> QQIEQPYR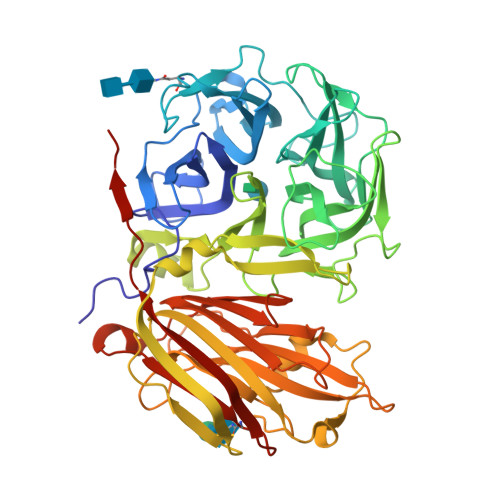TGYHFQPPSNWMNDPNGPMLYQGVYHFFYQYNPYAATFGDVIIWGHAVSYDLVNWIHLDPAIYPTQEADSKSCWSGSATILPGNIPAMLYTGSDSKSRQVQDLAWPKNLSDPFLREWVKHPKNPLITPPEGVKDDCFRDPSTAWLGPDGVWRIVVGGDRDNNGMAFLYQSTDFVNWKRYDQPLSSADATGTWECPDFYPVPLNSTNGLDTSVYGGSVRHVMKAGFEGHDWYTIGTYSPDRENFLPQNGLSLTGSTLDLRYDYGQFYASKSFFDDAKNRRVLWAWVPETDSQADDIEKGWAGLQSFPRALWIDRNGKQLIQWPVEEIEELRQNQVNLQNKNLKPGSVLEIHGIAASQADVTISFKLEGLKEAEVLDTTLVDPQALCNERGASSRGALGPFGLLAMASKDLKEQSAIFFRVFQNQLGRYSVLMCSDLSRSTVRSNIDTTSYGAFVDIDPRSEEISLRNLIDHSIIESFGAGGKTCITSRIYPKFVNNEEAHLFVFNNGTQNVKISEMSAWSMKNAKFVVDQSVKSAA>[15x]AEELLKRVEKL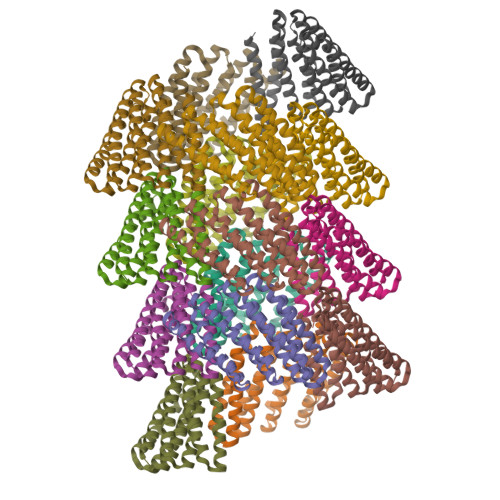VKEAEELLRQAMKKGSEELLEVALVVAQMAAREAKKVLTMAEVEGDPEVALRAVELVVRVAELLLRIALVSGSEEALERALRVAEEAARLAKRVLELAESQGDPEVALRAVELVVRVAELLLLIAKVSGSEEALERALRVAEEAARLAKRVLELAEKQGDPAVAILAVMLVKRVAELLENIARESGSEEAKERAERVREEARELQERVKELKERAG> EFAPSFDCGKPQVEPKKCPGRVVGGCVAHPHSWPWQVSLRTRFGMHFCGGTLISPEWVLTAAHCLEKSPRP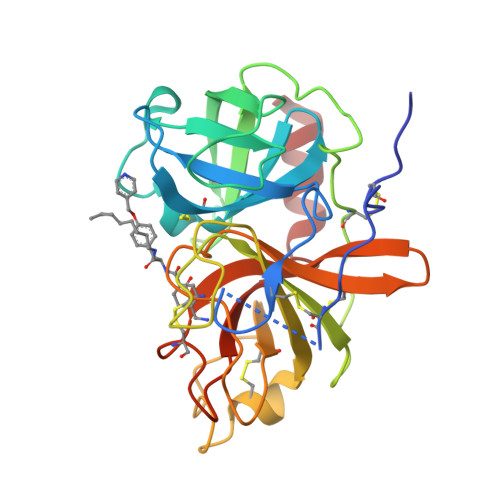SSYKVILGAHQEVNLEPHVQEIEVSRLFLEPTRKDIALLKLSSPAVITDKVIPACLPSPNYVVADRTECFITGWGETQGTFGAGLLKEAQLPVIENKVCNRYEFLNGRVQSTELCAGHLAGGTDSCQGDSGGPLVCFEKDKYILQGVTSWGLGCARPNKPGVYVRVSRFVTWIEGVMRNN Syntrophomonas wolfei is a syntrophic bacterium that is a leading model for examining how microbial communities degrade short-chain fatty acids. Syntrophomonas wolfei Göttingen uses acyl-CoA transferases to activate fatty acid substrates by synthesizing the respective CoA derivative. An acyl-CoA transferase paralog of particular interest is Act2 (Swol_0675). Act2 had numerous acylations and certain sites were modified by several different acyl groups.

To understand how these PTMs might affect the enzyme’s function, the structure of Act2, encoded by the gene Swol_0675, was determined by X-ray crystallography. The asymmetric unit of the tetragonal crystal lattice contains two molecules of Act2, which form a homodimeric structure. About 15% of the solvent accessible surface area of the monomer, or ~ 15,000 Å2, is buried in the intermolecular interface. Examination of crystal packing indicates that the Act2 homodimer likely forms a homotetramer mediated by a short β-strand-containing loop spanning residues Tyr127 to Asp140. A homotetrameric structure is consistent with the Act2 molecular mass estimated from size exclusion chromatography, with the computational prediction by the PISA webserver, and with existing acetyl-CoA transferase structures that also have a similar homotetrameric structures. The position of the four key catalytic residues (C91, N319, H357, C387) is virtually identical in all four of the structures as is the shielding of the active site by the covering (residues 146–161) and pantetheine loops (residues 246–250), which were identified in the human mitochondrial acetoacetyl- CoA thiolase (T2; Haapalainen et al., 2007). All the acyl-lysine sites identified in our proteomic datasets were mapped onto the S. wolfei Act2 structure and all are on the protein’s surface, with three sites located closer to the covering and pantetheine loop, K75, K208, and K233. The proximity of these modified lysine residues near the substrate tunnel suggest that these PTMs may be connected to the local buildup of RACS in this region. While the other modification sites are located on the enzyme’s surface but not near the substrate tunnel, these lysine residues could be involved in salt-bridge interactions that mediate tetramer formation. Out of these 5 sites, K75, K208, and K304 were located near the covering and pantetheine loops that surrounds the substrate tunnel, suggesting that these acyl modifications could affect substrate accessibility.

>[2x]SMAEINEVVVVGMARTPIGRYLGGLASVRANDLAIIAANAAIERAGVDPGIIDEIVGATCLHAGNGSLPPRIIGMKVGLPVRSGSCMVSQNCASGMRATEIACQNIMLGKTDISLVTAVESMSNIPYLLQQARSGYRMGDGKVQDAMLSDGLVCQLAGGHMGMTAENIAEKYGITREECDALALTSHQNAVKAVDEGIFDREIVPVVIKSKKGDKVISKDEHPIRGASLETMAKLPPAFKKGGVVTAANASGINDCAAAAVFMSKKKCEELGLKPLMKLVGICSEGVDAKVMGLGPAVAMPKVLKQAGWKYEDVDYWEVNEAFAAQVLGVVRMLKEEAGIELDFSKTNHNGSGIGLGHPVGATGLRIIVSMYYELERLGLTKGGASLCVGGGSAMASLWTRDI>[2x]EAASSSDADGKEVGSSGEGNRATGGKWRRPSLAQQRARRAQLPPAFDVVHWNDEDISRGHLLRVLHRDTFVVLDYHRQARMLTEEGNKAERVVS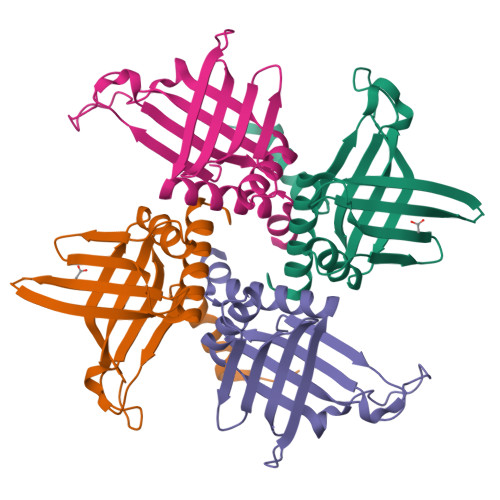VMLPAVYTARFLAVLEGRSEKVEVHSRYTNATFTPNPAAPYTFTLKCTSTRPAQQKQQVAGEEGDETFEWTVEFDVAESLMLQRFLTQALHYNTGFARTSV;>ASTFSGVQSLPKFEIHDVRDDPAEGTMTRVAVDGKLLLISQYPQLGPRKVDPNDLSPQFDADRRISVRLRHVDLAYLVGVCKERVPRHRMETKAYTLDFEKSAQGYHLHGKVHRVASQRMEDWSVKFDNHFAVTLEHFLESALDESFGFRQHYATRAAEGGEKIAATSSAEGGARRKRSVSDTSRYH[2x]>[3x]DNVEEGNHLYNAGKYQEALTFFMKPDAVNNPATMNRIGYMYDEGQGVKKDPKEAFKWYKKAADANLPVAQFNLGLMYQHGTGVSKDINES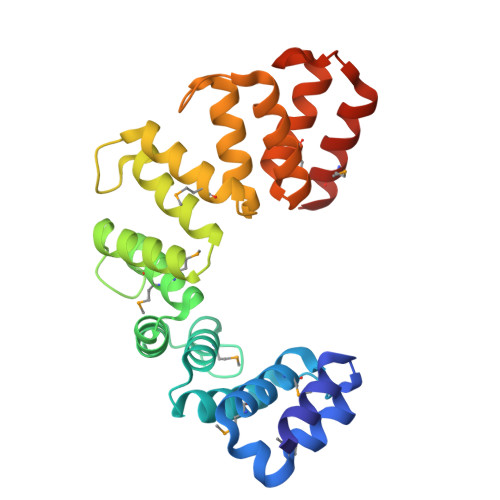IKWFRKAAEQNDPDAEMKMGYLTATGTGVKKDYQEAIQWYQRAAEHGDSAAYAQIGLFYTLGNGVKKDVNRAVQYYIMGAQKGDARAQAFLGKAYALGRGIQPDSEKALYWYKTAARNGNVNAMKELGSIYAKGRLGVKPDQQEAQRWNDMARKAEQKN> GSHMIKLTAQQ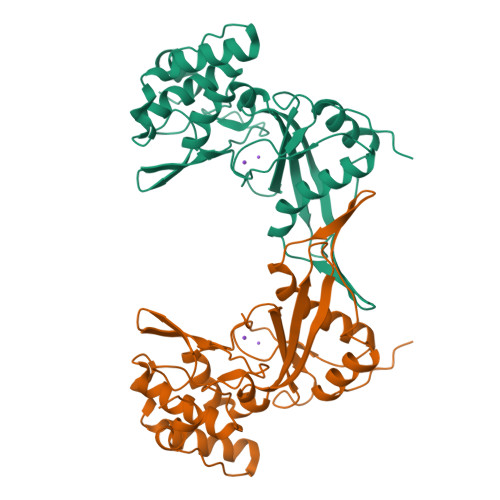IFDKLLDEEKILSANGQIRFFLGDVDIIVKQKDVVGNIIQEWLGGWLRKREIEFDVSTNTQMPPDFFLNKKDRSRELLEVKAFNRNASPGFDIADFKMYSDEIIHKPYMLDVDYLIFGYDMDDNGNVTIKDLWLKKVWQITRSMDGWAINLQVKKGVVHKIRPGVWYSINKKNMPMFECLEDFVSAIEETVYQNPATRHNASLWKRKFEEAYKKHYNRSISIPRWHEIAHKYKKK> IVGGTASVRGEWPWQVTLHTTSPTQRHLCGGSIIGNQWILTAAHCFYGVESPKILRVYSGILNQSEIKEDTSFFGVQEIIIHDQYKMAESGYDI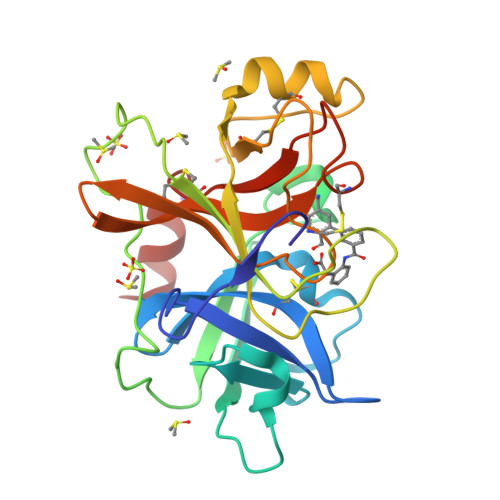ALLKLETTVNYTDSQRPISLPSKGDRNVIYTDCWVTGWGYRKLRDKIQNTLQKAKIPLVTNEECQKRYRGHKITHKMICAGYREGGKDACKGDAGGPLSCKHNEVWHLVGITSWGEGCAQRERPGVYTNVVEYVDWILEKTQAV> MSGIALSRLAQERKAWRKDHPFGFVAVPTKNPDGTMNLMNWECAIPGKKGTPWEGGLFKLRMLFKDDYPSSPPKCKFEPPLFHPNVYPSGTVCLSILEEDKDWRPAITIKQILLGIQELLNEPNIQDPAQAEAYTIYCQNRVEYEKRVRAQAKKFAPS;> MERREEQPGAAGAGAAPALDFTVENVEKALHQLYYDPNIENKNLAQKWLMQAQVSPQAWHFSWQLLQPDKVPEIQYFGASALHIKISRYWSDIPTDQYESLKAQLFTQITRFASGSKIVLTRLCVALASLALSMMPDAWPCAVADMVRLFQAEDSPVDGQGRCLALLELLTVLPEEFQTSRLPQYRKGLVRTSLAVECGAVFPLLEQLLQQPSSPSCVRQKVLKCFSSWVQLEVPLQDCEALIQAAFAALQDSELFDSSVEAIVNAISQPDAQRYVNTLLKLIPLVLGLQEQLRQAVQNGDMETSHGICRIAVALGENHSRALLDQVEHWQSFLALVNMIMFCTG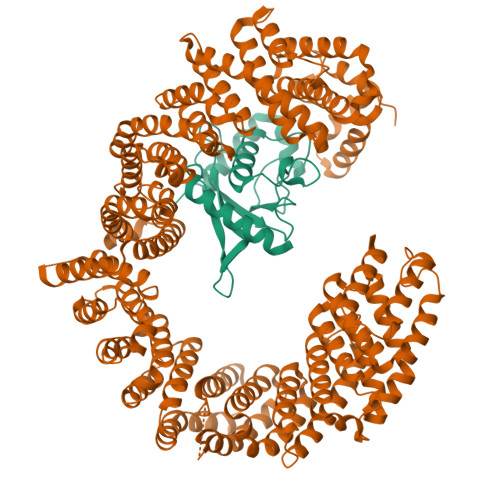IPGHYPVNETTSSLTLTFWYTLQDDILSFEAEKQAVYQQVYRPVYFQLVDVLLHKAQFPSDEEYGFWSSDEKEQFRIYRVDISDTLMYVYEMLGAELLSNLYDKLGRLLTSSEEPYSWQHTEALLYGFQSIAETIDVNYSDVVPGLIGLIPRISISNVQLADTVMFTIGALSEWLADHPVMINSVLPLVLHALGNPELSVSSVSTLKKICRECKYDLPPYAANIVAVSQDVLMKQIHKTSQCMWLMQALGFLLSALQVEEILKNLHSLISPYIQQLEKLAEEIPNPSNKLAIVHILGLLSNLFTTLDISHHEDDHEGPELRKLPVPQGPNPVVVVLQQVFQLIQKVLSKWLNDAQVVEAVCAIFEKSVKTLLDDFAPMVPQLCEMLGRMYSTIPQASALDLTRQLVHIFAHEPAHFPPIEALFLLVTSVTLTLFQQGPRDHPDIVDSFMQLLAQALKRKPDLFLCERLDVKAVFQCAVLALKFPEAPTVKASCGFFTELLPRCGEVESVGKVVQEDGRMLLIAVLEAIGGQASRSLMDCFADILFALNKHCFSLLSMWIKEALQPPGFPSARLSPEQKDTFSQQILRERVNKRRVKEMVKEFTLLCRGLHGTDYTADY>GPMAEKLNFEELNSMQRYSQFAVFRAIPGALGSDRAEIVAQAQSFFDGLETAGKVEVRGIYDLAGCRAEADFMIWWIAEEFEEIQAAFARFRRETVLGQVSEVAWLGNSLHRPAEFNRSHLPSFIMGEIPGDWITVYPFVRSYDWYIMDPQKRRKILAEHGQAARDFPDVRANTVPAFALGDYEYMLAFEAPRLDRIVDLMHKMRYTEARLHVREETPFFTGRRVSEVSELVNVLPG[5x]

ChdCs are enzymes involved in the prokaryotic heme biosynthesis pathway mainly of monoderm bacteria, but some diderm or intermediate representatives also use this pathway. They catalyze the hydrogen peroxide–driven oxidative decarboxylation of iron coproporphyrin III (coproheme) to iron protoporphyrin IX (heme b). After initial oxidation of coproheme to Compound I (two-electron deficient reaction intermediate), a catalytic tyrosine radical is generated, which is completely essential for both decarboxylation reactions. Mechanistic studies revealed the order of decarboxylation and proved that propionate at position 2 (p2) is decarboxylated first.

In this study, we designed variants where another tyrosine is introduced at the site of p4 (W183Y). A tyrosine residue is introduced as a potential radical site at the position of p4 in the active site in CdChdC W183Y. Also, we succeeded in solving the crystal structure of the W183Y variant, which allows evaluating the steric restraints around the newly introduced tyrosine residue. The structures clearly show that the introduced amino acids occupy the positions of the respective residues in the wild-type protein. While the distance between Y135 and Cß-p2 is about 3.1 Å in the wild-type structure, the Y183 oxygen lies about 4.4 Å above the Cß of p4. Both single mutations leave the active site and the overall structure is unaffected. Introducing a second potential catalytic tyrosine in the W183Y variant, spectral features very similar to the wild-type protein are observable. While the characteristic shape of the CdChdC Soret maximum is slightly altered (393 nm with a less pronounced shoulder at 373 nm), the characteristic spectral shift of the Soret maximum upon addition of H2O2 is observed even to 406 nm. The introduction of another tyrosine in close proximity to the redox-active substrate leads to approximately 11% nitrosylation on Y183 and 50% radical formation on Y135. Compared to the wild-type protein this is even an increase in nitrosylated Y135, which can be explained by a hampered reaction and slight accumulation of Compound I* in the variant.>[2x]GSFTMPSPQLLVLFGSQT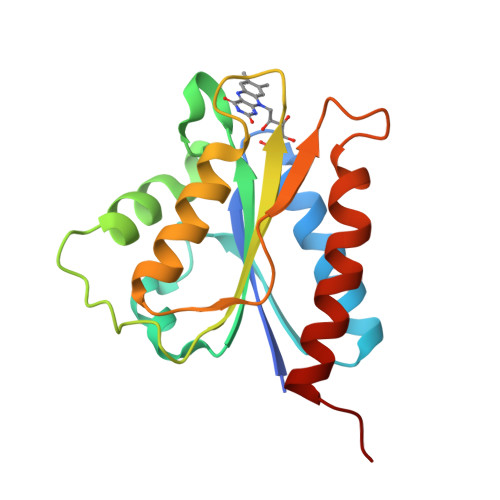GTAQDVSERLGREARRRRLGCRVQALDSYPVVNLINEPLVIFVCATTGQGDPPDNMKNFWRFIFRKNLPSTALCQMDFAVLGLGDSSYAKFNFVAKKLHRRLLQLGGSALLPVCLGDDQHELGPDAAVDPWLRDLWDRVLGLYPPPP Toll-like Receptor 3 (TLR3) plays a key role in anti-viral defenses by inducing a potent immune response against double-stranded RNAs (dsRNAs) produced by viral infection. Previous crystallographic studies show that RNA ligand binds to the extracellular domains of TLR3 and induces the formation of a homodimer of TLR326. The charge interaction with the phosphate backbone of the RNA double helix plays the principal role in the interaction. The ligand-binding site involves both the N and C-terminal parts of the TLR3 ectodomain.

To determine whether the transmembrane and intracellular domains are necessary for the linear clustering of TLR3, we produced the ectodomain of TLR3 (ectoTLR3) and determined its structure in complex with poly(I:C) dsRNA. To study the cooperativity of the clustering, we titrated the ratio of ectoTLR3 molecules against the number of available binding sites in the poly(I:C). Even in the most poly(I:C) excess condition, the electron microscopic images show that a significant portion of the TLR3 particles still is in the clustered state along the dsRNA. In the subsequent 2D classification analysis, the number of the TLR3 particles in the cluster was estimated to be 50% of those in the dimeric state. In a close inspection of the micrographs, we found that almost all of the particles bound to the straight double-helical part of the dsRNA are in the clustered state. The vast majority of TLR3 not in the clustered state is located either where the TLR3 clusters ended or where the RNA strands make irregular kinks. This observation demonstrates that clustering is a dominant feature for TLR3 when bound to RNAs with regular double-helical structures.

>ADPKCTVSHEVADCSHLKLTQVPDDLPTNITVLNLTHNQLRRLPAANFTRYSQLTSLDVGFNTISKLEPELCQKLPMLKVLNLQHNELSQLSDKTFAFCTNLTELHLMSNSIQKIKNNPFVKQKNLITLDLSHNGLSSTKLGTQVQLENLQELLLSNNKIQALKSEELDIFANSSLKKLELSSNQIKEFSPGCFHAIGRLFGLFLNNVQLGPSLTEKLCLELANTSIRNLSLSNSQLSTTSNTTFLGLKWTNLTMLDLSYNNLNVVGNDSFAWLPQLEYFFLEYNNIQHLFSHSLHGLFNVRYLNLKRSFTKQSISLASLPKIDDFSFQWLKCLEHLNMEDNDIPGIKSNMFTGLINLKYLSLSNSFTSLRTLTNETFVSLAHSPLHILNLTKNKISKIESDAFSWLGHLEVLDLGLNEIGQELTGQEWRGLENIFEIYLSYNKYLQLTRNSFALVPSLQRLMLRRVALKNVDSSPSPFQPLRNLTILDLSNNNIANINDDMLEGLEKLEILDLQHNNLARLWKHANPGGPIYFLKGLSHLHILNLESNGFDEIPVEVFKDLFELKIIDLGLNNLNTLPASVFNNQVSLKSLNLQKNLITSVEKKVFGPAFRNLTELDMRFNPFDCTCESIAWFVNWINETHTNIPELSSHYLCNTPPHYHGFPVRLFDTSSCKSGRLVPRGSHHHHHH[2x]> AVIGMNEAASALTPSRVSSLPDTQRAAWQEYLARSEAQLSRDKASLAAELAPGQPLPPPPAEGKGADTMPLDKPAAWYTSKAARHVADVIVSFQTPAGGWGKNQPRDGALRLPGQHYTGENVAKVKSGSNDLDAARDRDWHYVGTIDNDATVTEIRFLAQVVSQLAPEEAAPYRDAALKGIEYLLASQFPNGGWPQVWPLEGGYHDAITYNDDALVHVAELLSDIAAGRDGFGFVPPAIRTRALEATNAAIHCIVETQVVQDGKRLGWGQQHDALTLRPTSARNFEPAALSSTESARILLFLMEIEAPSDAVKQAIRGGVAWLNTSVIRDRAWVKSDQGYQLVTEQGAKPLWSRFYSLDGN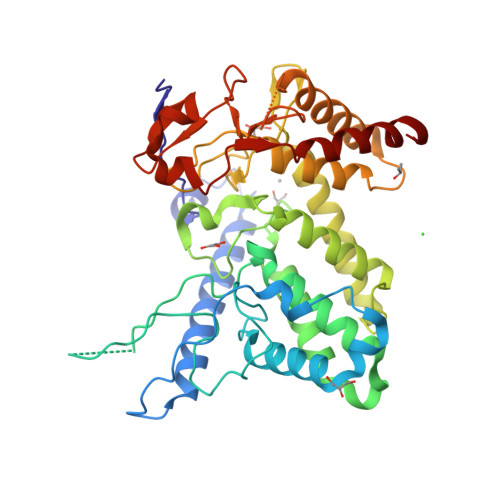KPVFGDRDKTIHDDVMGISQERRTGYAWYTTSPQKALSAFTKWEKRS> MPPGVDCPMEFWTKEENQSVVVDFLLPTGVYLNFPVSRNANLSTIKQLLWHRAQYEPLFHMLSGPEAYVFTCINQTAEQQELEDEQRRLCDVQPFLPVLRLVAREGDRVKKLINSQISLLIGKGLHEFDSLCDPEVNDFRAKMCQFCEEAAARRQQLGWEAWLQYSFPLQLEPSAQTWGPGTLRLPNRALLVNVKFEGSEESFTFQVSTKDVPLALMACALRKKATVFRQPLVEQPEDYTLQVNGRHEYLYGSYPLCQFQYICSCLHSGLTPHLTMVHSSSILAMRDEQSNPAPQVQKPRAKPPPIPAKKPSSVSLWSLEQPFRIELIQGSKVNADERMKLVVQAGLFHGNEMLCKTVSSSEVSVCSEPVWKQRLEFDINICDLPRMARLCFALYAVIEKAKKARSTKKKSKKADCPIAWANLMLFDYKDQLKTGERCLYMWPSVPDEKGELLNPTGTVRSNPNTDSAAALLICLPEVAPHPVYYPALEKILELGRHSECVHVTEEEQLQLREILERRGSGELYEHEKDLVWKLRHEVQEHFPEALARLLLVTKWNKHEDVAQMLYLLCSWPELPVLSALELLDFSFPDCHVGSFAIKSLRKLTDDELFQYLLQLVQVLKYESYLDCELTKFLLDRALANRKIGHFLFWHLRSEMHVPSVALRFGLILEAYCRGSTHHMKVLMKQGEALSKLKALNDFVKLSSQKTPKPQTKELMHLCMRQEAYLEALSHLQSPLDPSTLLAEVCVEQCTFMDSKMKPLWIMYSNEEAGSGGSVGIIFKNGDDLRQDMLTLQMIQLMDVLWKQEGLDLRMTPYGCLPTGDRTGLIEVVLRSDTIANIQLNKSNMAATAAFNKDALLNWLKSKNPGEALDRAIEEFTLSCAGYCVATYVLGIGDRHSDNIMIR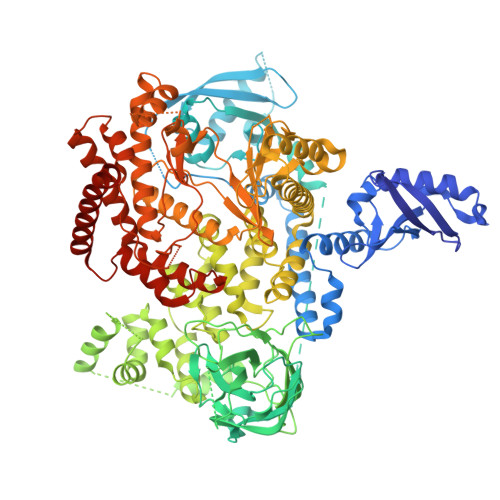ESGQLFHIDFGHFLGNFKTKFGINRERVPFILTYDFVHVIQQGKTNNSEKFERFRGYCERAYTILRRHGLLFLHLFALMRAAGLPELSCSKDIQYLKDSLALGKTEEEALKHFRVKFNEALRESWKTKVNWLAHNVSKDNRQ> MRSTQEERFEQRIAQETAIEPQDWMPDAYRKTLIRQIGQHAHSEIVGMLPEGN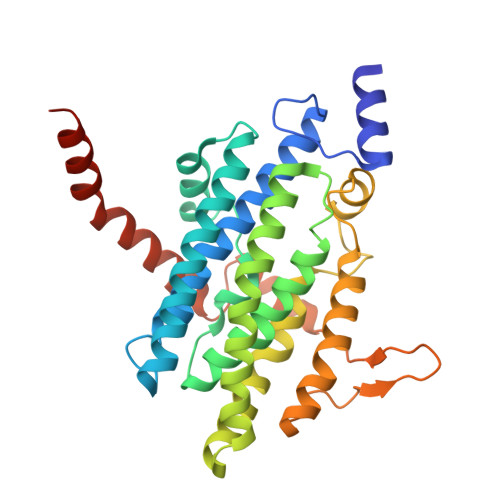WITRAPTLRRKAILLAKVQDEAGHGLYLYSAAETLGCAREDIYQKMLDGRMKYSSIFNYPTLSWADIGVIGWLVDGAAIVNQVALCRTSYGPYARAMVKICKEESFHQRQGFEACMALAQGSEAQKQMLQDAINRFWWPALMMFGPNDDNSPNSARSLTWKIKRFTNDELRQRFVDNTVPQVEMLGMTVPDPDLHFDTESGHYRFGEIDWQEFNEVINGRGICNQERLDAKRKAWEEGTWVREAALAHAQKQHARKVA>[6x]GEEL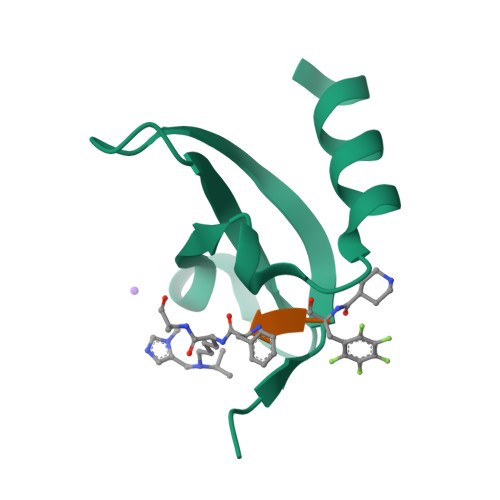YEVERIVDKRKNKKGKTEYLVRWKGYDSEDDTWEPEQHLVNCEEYIHDFNRRH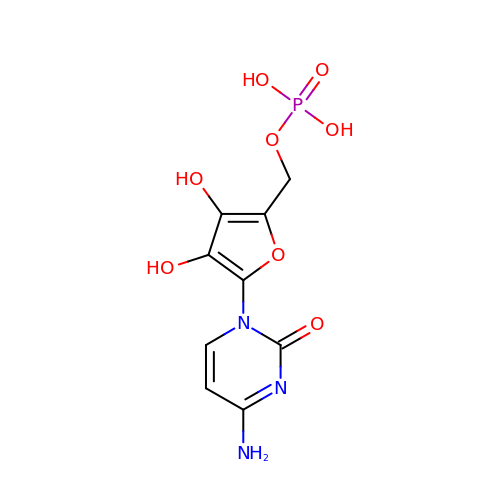[5-(4-azanyl-2-oxidanylidene-pyrimidin-1-yl)-3,4-bis(oxidanyl)furan-2-yl]methyl dihydrogen phosphate | C9 H10 N3 O8 P | KCVPKYRTVHKUFJ-UHFFFAOYSA-N> APYCV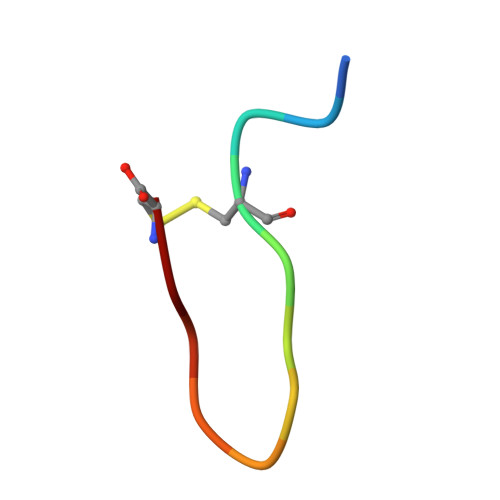YRGSWSC> APSQEEAVIAFGKFKLNLGTREMFREDEPMPLTSGEFAVLKALVSHPREPLSRDKLMNLARGREYSAMERSIDVQISRLRRMVEEDPAHPRYIQTVWGLGYVFVPDG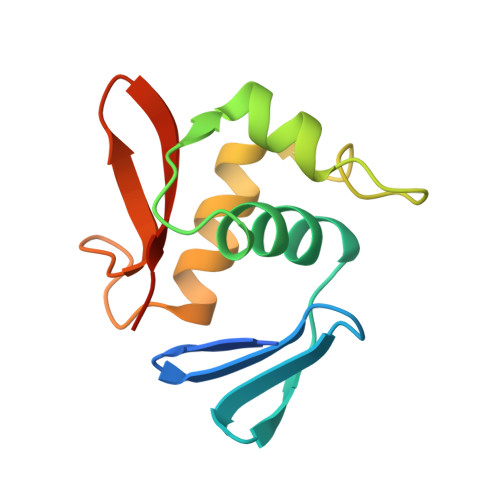SKA>MHHHHHGAASMSNTTLHATTIYAVRHNGKAAMAGDGQVTLGQQVIMKQTARKVRRLYEGKVLAGFAGSVADAFTLFEKFETKLQQFSGNL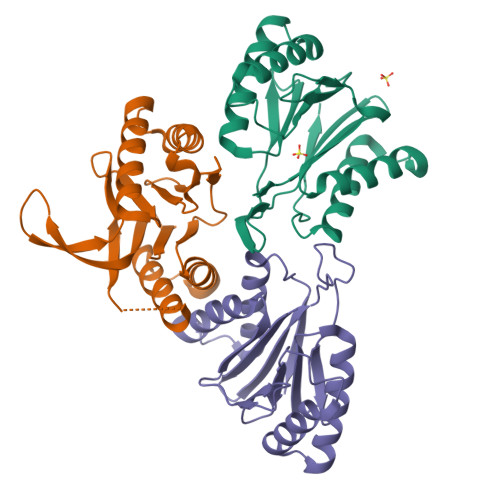ERAAVELAQEWRGDKQLRQLEAMLIVMDKDAILVVSGTGEVIAPDDDLIAIGSGGNYALSAGRALKRHASHLSAEEMAYESLKVAADICVFTNDNIVVETL[12x]>AKVTMLYVPCTINQVLVKAFVDSGAQNSIMNKRTAERCGLMRLVDVRMRGVAVGVGRQEICGRIHMTPVNLAGMYIPFAFYVIEDQAMDLIIGLDQLKRHQMMIDLKH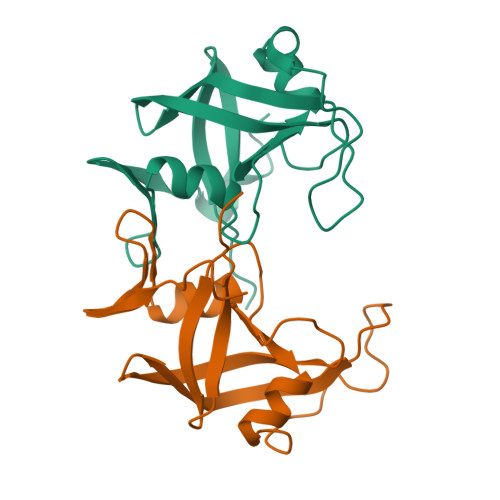NCLTIDNINVPFLPENDLPALA[4x]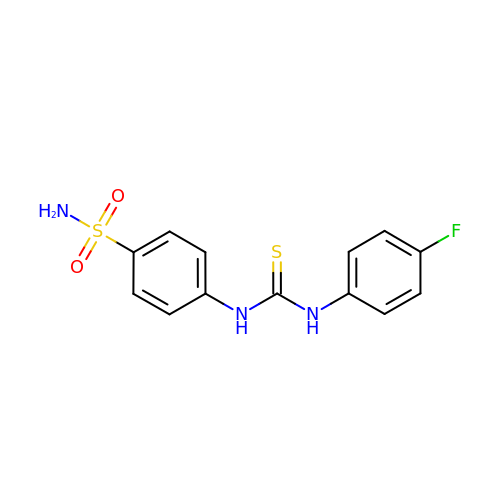4-{[(4-fluorophenyl)carbamothioyl]amino}benzene-1-sulfonamide | C13 H12 F N3 O2 S2 | VUDOFEJVAFMLEC-UHFFFAOYSA-N> MSEPMMWLLVRGVWETLAMTFVSGFFGFVIGLPVGVLLYVTRPGQIIANAKLYRTVSAIVNIFRSIPFIILLVWMIPFTRVIVGTSIGLQAAIVPLTVGAAPFIARMVENALLEIPTGLIEASRAMGATPMQIVRKVLLPEALPGLVNAATITLITLVGYSAMGGAVGAGGLGQIGYQYGYIGYNATVMNTVLVLLVILVYLIQFAGDRIVRA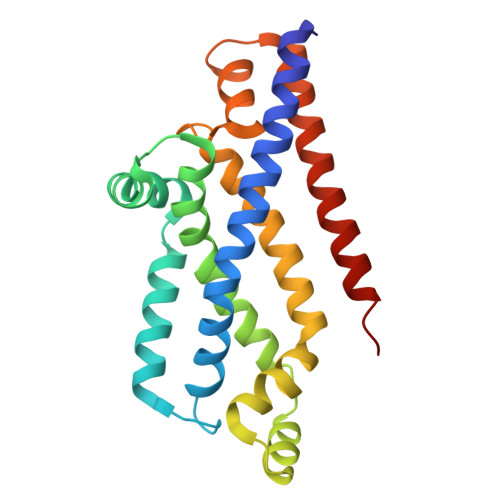VTRK> MIREGDKVVLVDPRGKRYLITVSKRDFHTDLGILKLEEIIGRNFGEAIKSHKGHEFKILRPRIVDYLDKMKRGPQIVHPKDAALIVAYAGISPGDFIVEAGVGSGALTLFLANIVGPEGRVVSYEIREDFAKLAWENIKWAGFDDRVTIKLKDIYEGIEEENVDHVILDLPQPERVVEHAAKALKPGGFFVAYTPCSNQVMRLHEKLREFKDYFMKPRTINVLVFDQEVKKECMRPRTTALVHTGYIT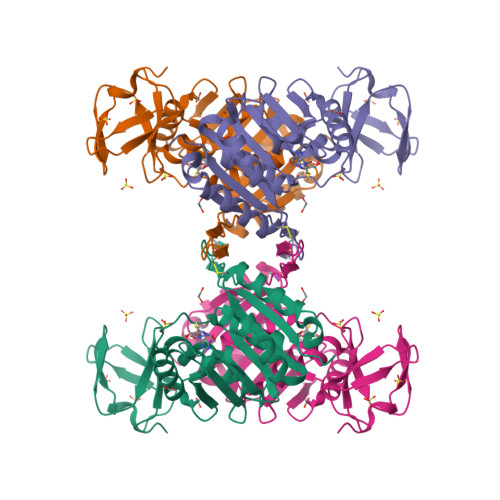FARRILE>MADLAESNIKVMCRFRPLNESEVNRGDKYIAKFQGEDTVVIASKPYAFDRVFQSSTSQEQVYNDAAKKIVKDVLEGYNGTIFAYGQASSGKTHTMEGKLHDPEGMGIIPRIVQDIFNYIYSMDENLEFHIKVSYF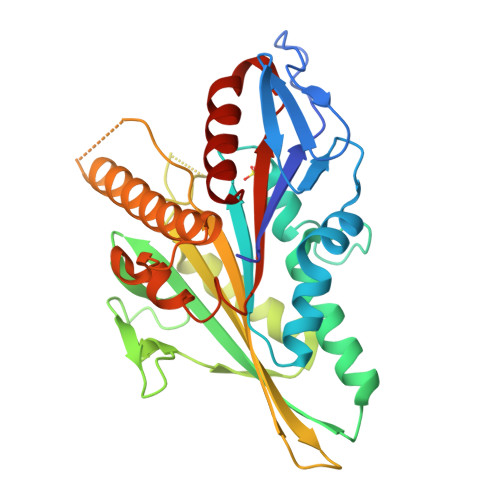EIYLDKIRDLLDVSKTNLSVHEDKNRVPYVKGATERFVSSPDEVMDTIDEGKSNRHVAVTNMNEHSSRSHSIFLINVKQENTQTEQKLSGKLYLVDLAGSEKVSKTGAEGAVLDEAKNINKSLSALGNVISALAEGSTYVPYRDSKMTRILQDSLGGNARTTIVICCSPSSYNESETKSTLLFGQRAKTI[6x]> SATTGARSASVGWAESLIGLHLGKVAL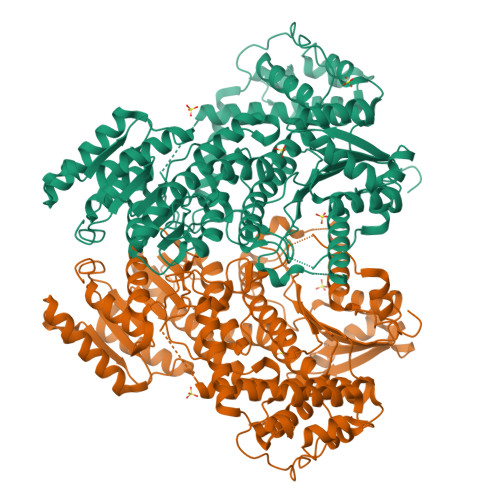ITGGSAGIGGQIGRLLALSGARVMLAARDRHKLEQMQAMIQSELAEVGYTDVEDRVHIAPGCDVSSEAQLADLVERTLSAFGTVDYLINNAGIAGVEEMVIDMPVEGWRHTLFANLISNYSLMRKLAPLMKKQGSGYILNVSSYFGGEKDAAIPYPNRADYAVSKAGQRAMAEVFARFLGPEIQINAIAPGPVEGDALRGTGERPGLFARRARLILENKRLNELHAALIAAARTDERSMHELVELLLPNDVAALEQNPAAPTALRELARRFRSEGDPAASSSSALLNRSIAAKLLARLHNGGYVLPADIFANLPNPPDPFFTRAQIDREARKVRDGIMGMLYLQRMPTEFDVAMATVYYLADRNVSGETFHPSGGLRYERTPTGGELFGLPSPERLAELVGSTVYLIGEHLTEHLNLLARAYLERYGARQVVMIVETETGAETMRRLLHDHVEAGRLMTIVAGDQIEAAIDQAITRYGRPGPVVCTPFRPLPTVPLVGRKDSDWSTVLSEAEFAELCEHQLTHHFRVARKIALSDGASLALVTPETTATSTTEQFALANFIKTTLHAFTATIGVESERTAQRILINQVDLTRRARAEEPRDPHERQQELERFIEAVLLVTAPLPPEADTRYAGRIHRGRAITV>MGFLSGKRILVTGVASKLSIAYGIAQAMHREGAELAFTYQNDKLKGRVEEFAAQLGSDIVLQCDVAEDASIDTMFAELGKVWPKFDGFVHSISFAPGDQLDGDYVNAVTREGFKIAHDISSYSFVAMAKACRSMLNPGSALLTLSYLGAERAIPNYNVMGLAKASLEANVRYMANAMGPEGVRVNAISAGPIRTLAASGIKDFRKMLAHCEAVTPIRRTVTIEDVGNSAAFLCSDLSAGISGEVVHVDGGFSI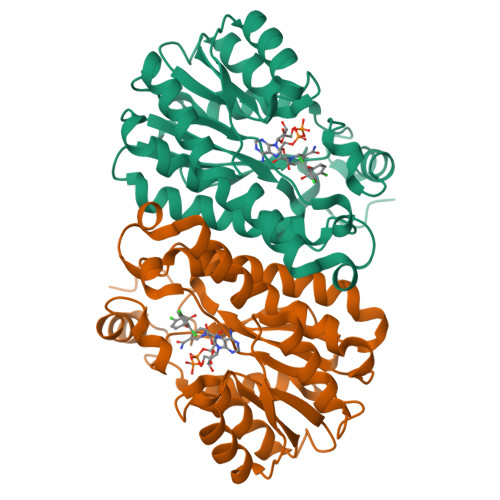AAMNELELKLEHHHHHH[2x]>[2x]MMTLNRKCVVIHNGSHRTVAGFSNVELPQCIIPSSYIKRTDEGGEAEFIFGTYNMIDAAAEKRNGDEVYTLVDSQGLPYNWDALEMQWRYLYDTQLKVSPEELPLVITMPATNGKPDMAILERYYELAFDKLNVPVFQIVIEPLAIALSMGKSSAFVIDIGASGCNVTPIIDGIVVKNAVVRSKFGGDFLDFQVHERLAPLIKEENDMENMADEQKRSTDVWYEASTWIQQFKSTMLQVSEKDLFELERYYKEQADIYAKQQEQLKQMDQQLQYTALTGSPNNPLVQKKNFLFKPLNKTLTLDLKECYQFAEYLFKPQLISDKFSPEDGLGPLMAKSVKKAGASINSMKANTSTNPNGLGTSHINTNVGDNNSTASSSNISPEQVYSLLLTNVIITGSTSLIEGMEQRIIKELSIRFPQYKLTTFANQVMMDRKIQGWLGALTMANLPSWSLGKWYSKEDYETLKRDRKQSQATNATNLVPRGSHHHHHH;>MAPFRQDSILIIYPRSQTTLVQFGLNEETFTVPELEIPTQIYRTTRQDGSYTYHSTNKDNKAELIKPIQNGEIIDISAFTQFLRLIFVSILSDRANKNQDAFEAELSNIPLLLITHHSWSQSDLEIITQYVFESLEINNLIQLPASLAATYSMISLQNCCIIDVGTHHTDIIPIVDYAQLDHLVSSIPMGGQSINDSLKKLLPQWDDDQIESLKKSPIFEVLSDDAKKLSSFDFGNENEDEDEGTLNVAEIITSGRDTREVLEERERGQKVKNVKNSDLEFNTFWDEKGNEIKVGKQRFQGCNNLIKNISNRVGLTLDNIDDINKAKAVWENIIIVGGTTSISGFKEALLGQLLKDHLIIEPEEEKSKREEEAKSVLPAATKKKSKFMTNSTAFVPTIEYVQCPTVIKLAKYPDYFPEWKKSGYSEIIFLGAQIVSKQIFTHPKDTFYITREKYNMKGPAALWDVQF[2x];>[2x]SMDPQTLITKANKVSYYGNPTSKESWRYDWYQPSKVSSNVQQPQQQLGDMENNLEKYPFRYKTWLRNQEDEKNLQRESCEDILDLKEFDRRILKKSLMTSHTKGDTSKATGAPSANQGDEALSVDDIRGAVGNSEAIPGLSAGVNNDNTKESKDVKMN

Chromatin-remodeling complexes (remodelers) are large, multisubunit complexes that regulate gene expression and genome maintenance. The HSA domain of Sth1, the catalytic subunit of the budding yeast SWI/SNF-family remodeler RSC (Remodeling the Structure of Chromatin), recruits Arp7 and Arp9. In turn, the Arp7/9 heterodimer forms a tight complex with another auxiliary subunit, Rtt102. Arp7/9 regulates the nucleosome sliding, ejection, and ATPase activities of RSC in an Rtt102-dependent manner.

Here, we pre-incubated Rtt102-Arp7/9 with ATP prior to crystallization, and obtained crystals using polyethylene glycol 3350 as the main precipitant. The crystals, which diffracted to a relatively low resolution (3.25 Å), contain two copies of the Rtt102-Arp7/9 ternary complex in the P1 unit cell (RMSD = 0.51 Å for 833 equivalent Cα atoms). The conformation of Rtt102 is also very similar to that observed in the complex of Rtt102-Arp7/9-HSA, and, although the current structure reveals 13 more amino acids for this subunit, a large portion of Rtt102 (90 amino acids out of 157) remains unresolved in the electron density map. More importantly, unlike in previous structures, composite omit maps of the current structure clearly showed the presence of ATP in the nucleotide-binding cleft of Arp7 but not Arp9 in both complexes of the unit cell. A nucleotide-bound structure of Rtt102-Arp7/9 reveals that ATP binds only to Arp7, helping stabilize a closed conformation of Arp7 that potentiates binding of Rtt102-Arp7/9 to the HSA domain. Not surprisingly, we found here that Arp7 lacks ATPase activity, both alone and within the ternary complex Rtt102-Arp7/9, whereas the quaternary complex Rtt102-Arp7/9-Sth1301–1097 displays strong DNA-dependent ATPase activity catalyzed by subunit Sth1. In particular, the all-important actin residue Lys-18, which anchors the nucleotide in place by interacting with both the α-phosphate and β-phosphate, becomes Val-18 in Arp7, which cannot support these interactions. In contrast, there is no cation associated with the nucleotide in the structure of Arp7. Indeed, Arp7 appears to lack a cation-binding site, as two of the residues that coordinate water molecules that hold the cation in place in actin, Asp-11 and Gln-137, have changed in Arp7 to His-11 and Glu-141, respectively. In summary, the biochemical and structural data presented here suggest that Rtt102 and ATP stabilize a conformation of Arp7/9 that potentiates binding to the HSA domain, which in turn releases intramolecular interactions between the pHSA domain and the P1 region of the ATPase domain.> MDVPADSHIKYEDAIDYWTDVDATVDGVLGGYGEGTVVPTMDVLGSNNFLRKLKSRMLPQENNVKYAVDIGAGIGRVSKTMLHKHAAKIDLVEPVKPFIEQMHVELAELKDKGQIGQIYEVGMQDWTPDAGKYWLIWCQWCVGHLPDAELVAFLKRCIVGLQPNGTIVVKENNTPTDTDDFDETDSSVTRSDAKFRQI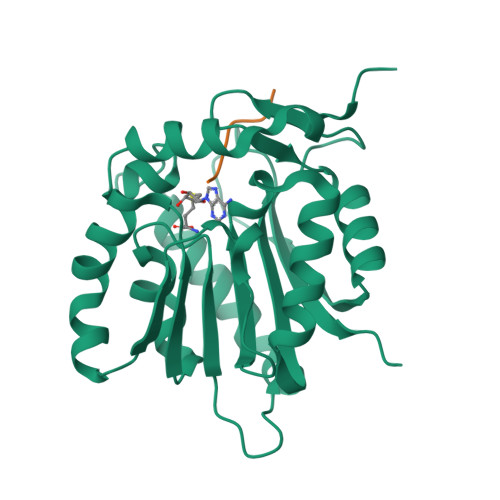FEEAGLKLIASERQRGLPRELYPVRMYALKPMPN;> PPKQQL> SAYSTREILLALCIRDSRVHGNGTLHPVL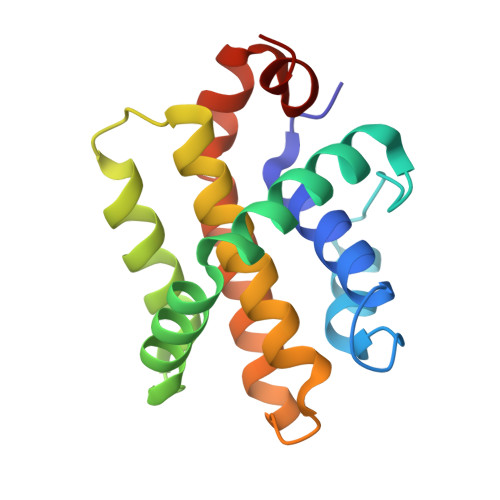ELAARETPLRLSPEDTVVLRYHVLLEEIIERNSETFTETWNRFITHTEHVDLDFNSVFLEIFHRGDPSLGRALAWMAWCMHACRTLCCNQSTPYYVVDLSVRGMLEASEGLDGWIHQQGGWSTLIEDNI>MVRKGEKKLAKPATTKAANPQPRRRANNRRRSNRTDAPVSKASTVTGFGRGTNDVHLSGMSRISQAVLPAGTGTDGYVVVDATIVPDLLPRLGHAARIFQRYAVETLEFEIQPMCPANTGGGYVAGFLPDPTDNDHTFDALQATRGAVVAKWWESRTVRPQYTRTLL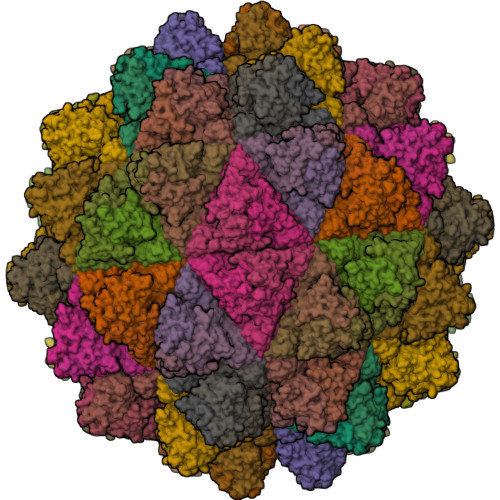WTSSGKEQRLTSPGRLILLCVGNNTDVVNVSVLCRWSVRLSVPSLENPEETTAPIMTQGSLYNDSLSTNDFKSILLGSTPLDIAPDGAVFQLDRPLSIDYSLGTGDVDRAVYWHLKKFAGNAGTPAGWFRWGIWDNFNKTFTDGVAYYSDEQPRQILLPVGTVCTRVDSEN[90x]>[2x]METFEISDFKEHAKKKSMWAGALNKVTISGLMGVFTEDEDLMALPIHRDHCPALLKIFDELIVNATDHERACHNKTKKVTYIKISFDKGVFSCENDGPGIPIVKHEQASLIAKRDVYVPEVASCYFLAGTNINKAKDCIKGGTNGVGLKLAMVHSQWAILTTADGSQKYVQHINQRLDNIEPPTITPSREMFTRIELMPVYQELGYAQPLSETEQADLSAWIYLRACQCAAYVGKGTTIYYNDKPCSTSSVMALAKMYTLVTAPNSTIYTATIKADAKPYSLHPLQVAAVVSPKFKKFEHVSIINGVNCVKGEHVTFLKKAINEMVVKK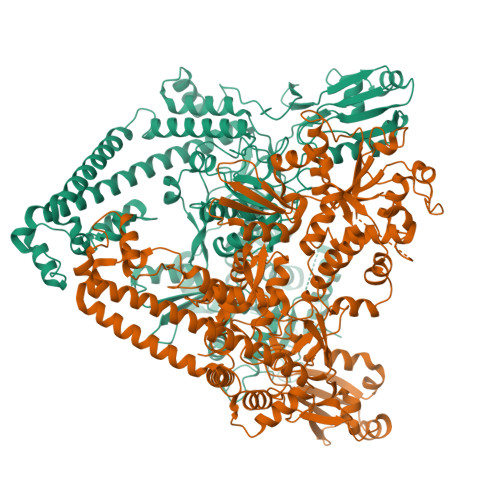FQQTIKDKNRKTTLRDSCSNIFVVIVGSIPGIEWTGQRKDELSIAENVFKTHYSIPSSFLTSMTRSIVDILLQSISKKDNHKQIDVDKYTRARNAGGKKAQDCMLLAAEGDSALSLLRAGLTLGKSNPSGPSFDFCGMISLGGVIMNACKKVTNITTDSGETIMVRNEQLTNNKVLQGIVQVLGLDFNCHYKTQEERAKLRYGCIVACVDQDLDGCGKILGLLLAYFHLFWPQLIVHGFVKRLLTPLIRVYEKGNTVPVEFYYEQEFDAWAKKQTSLANHTVKYYKGLAAHDTHEVKSMFKHFDKMVYTFTLDDSAKELFHIYFGGESELRKRELCTGVVPLTETQTQSIHSVRRIPCSLHLQVDTKAYKLDAIERQIPNFLDGMTRARRKILAGGLKCFASNNRERKVFQFGGYVADHMFYHHGDMSLNTSIIKAAQYYPGSSHLYPVFIGIGSFGSRHLGGKDAGSPRYISVQLASEFIKTMFPTEDSWLLPYVFEDGQRAEPEYYVPVLPLAIMEYGANPSEGWKYTTWARQLEDILALVRAYVDKNNPKHELLHYAIDHKITVLPLRPSNYNFKGHLKRFGQYYYSYGTYVVSEQRNMITITELPLRVPTVAYIESIKKSSNRMAFIEEIVDYSSSETIEILVKLKPNSLSRIMEEFKETEEQNSIENFLRLRNCLHSHLNFVKPKGGIIEFNSYYEILYAWLPYRRDLYQKRLMRERAVLKLRLIMETAIVRYINESADLNLSHYEDEKEAGRILSEHGFPPLNQSLITSPEFATIEELNQKALQGCYTYILSLQARELLIAAKTRRVEKIKKMQARLDKVEQLLQESPFPGASVWLEEIDAVEKAIIKGRNTQWKFH>MGHHHHHHSSGRENLYFQGMAYDLWYWDGIPGRGEFVRLALEAGKIPYRD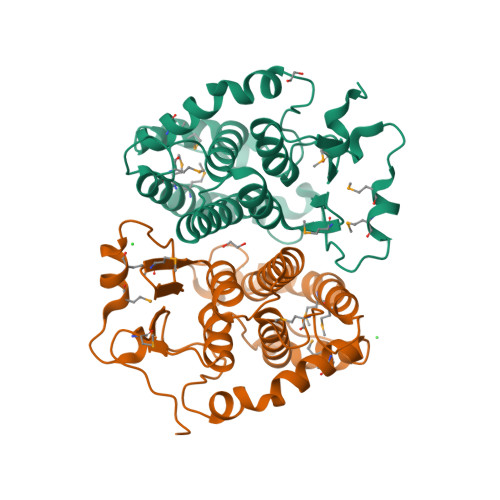RAREPGEDMLDDMRRRRDTPPFAPPYLVADGMTIAQTANILLFLGVEHGLAPPDRAGRLWVNQLQLTIADLTAEAHDVHHPVAAGLYYEDQQDVALRRAADFRETRMPKFMQYFEQALDRPGGWLTDMGRWSYADLSLYHVVEGLLHAFPRRMRTLVHRYPRLMALHARVAELPELRGYLASDRRLPFGDGIFRHYPELDGA[2x]> SKYVDRVIAEVEKKYADEPEFVQTVEEVLSSLGPVVDAHPEYEEVALLERMVIPERVIEFRVPWEDDNGKVHVNTGYRVQFNGAIGPYLG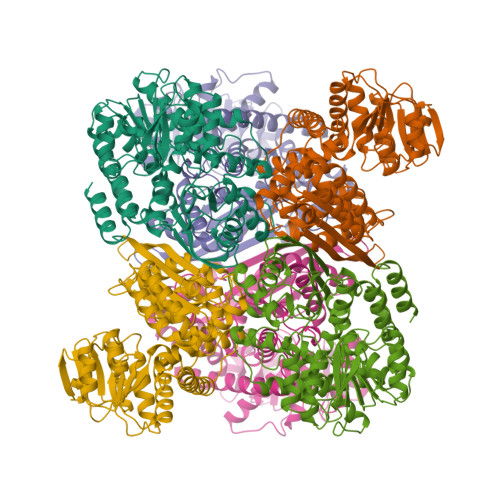GLRFAPSVNLSIMKFLGFEQAFKDSLTTLPMGGAKGGSDFDPNGKSDREVMRFCQAFMTELYRHIGPDIDVPAGDLGVGARELGYMYGQYRKIVGGFYNGVLTGKARSFGGSLVRPEATGYGSVYYVEAVMKHENDTLVGKTVALAGFGNVAWGAAKKLAELGAKAVTLSGPDGYIYDPEGITTEEKINYMLEMRASGRNKVQDYADKFGVQFFPGEKPWGQKVDIIMPCATQNDVDLEQAKKIVANNVKYYIEVANMPTTNEALRFLMQQPNMVVAPSKAVNAGGVLVSGFEMSQNSERLSWTAEEVDSKLHQVMTDIHDGSAAAAERYGLGYNLVAGANIVGFQKIADAMMAQGIAW> GCPTLYTPGSGQFLTTDDFQTPCMLPKFQPTPVIDIPGEVKNFLEVIQVESLVEINNVSGVEGVARYRIPLNV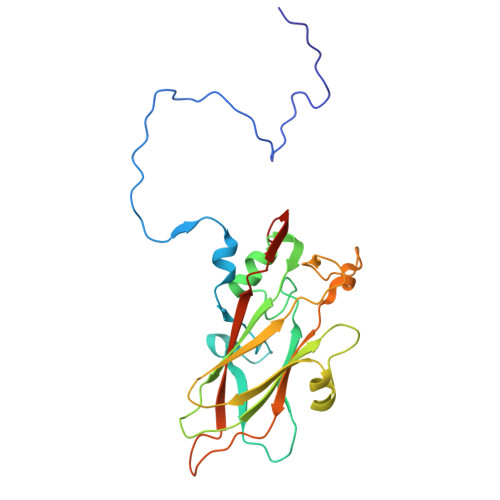QDAMDGQIMAVRVDPGADGPMQSTLLGVFTRYYTQWSGSLDFTFMFCGTFMTTGKVIIAYTPPGGDQPGSRQQAMLGTHVVWDFGLQSSITLVVPWISSGHFRGTSLDNTIYKYRYYEAGYITMWYQTNMVVPPNFPTEASILMFVAAQPNFSLRILKDRPDITQVASLQ> GSQAPVYGERLEGFDYAYPVHYLDFTSQGQPLSMAYLD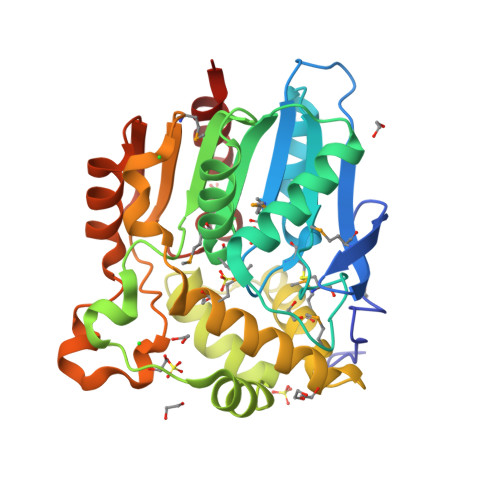VAPKKANGRTILLMHGKNFCAGTWERTIDVLADAGYRVIAVDQVGFCKSSKPAHYQYSFQQLAANTHALLERLGVARASVIGHSMGGMLATRYALLYPRQVERLVLVNPIGLEDWKALGVPWRSVDDWYRRDLQTSAEGIRQYQQATYYAGEWRPEFDRWVQMQAGMYRGKGRESVAWNSALTYDMIFTQPVVYELDRLQMPTLLLIGEKDNTAIGKDAAPAELKARLGNYAQLGKDAARRIPQATLVEFPDLGHTPQIQAPERFHQALLEGLQTQP>MSLTKLYYEDQYIKEFKGEIIEVKEIDGKFHVLLDQTAFFPGGGGQMGDLGLIDGIKVLDVYEEEGKVYHVLEKEPKKLKNLQCELDWERRFDGMQQHLGQHLLSGCFYDLFGANTCGFHLGKEISTVDIVGFLDEKTIREAEKEANRLIFENLEVKSYAPSKKELKKVKTRRALPKTDEEIRIVEIVGLDLN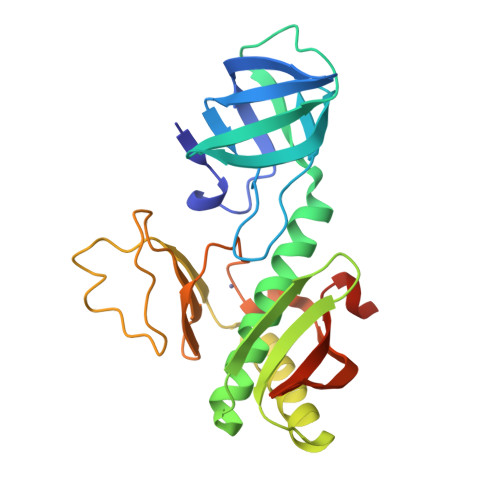ACCGVHPRNTRDLQVIKIRRWEKHKNATRIEYVAGNRAVSEGHHHHHH[2x]> MASVIKPTQYKPVPDEEPNSTDVEETLERIKNNDPKLEEVNLNNIRNIPIPTLKAYAEALKENSYVKKFALANTRADDHVAFAIAIMLKANKTITSLNLDSNHITGKGILAIFRALLQNNTLTELRFHNQRHICGGKTEMEIAKLLKENTTLLKLGYHFELAGPRMTVTNLLSRNMDKQRQKRLQEQRQAQ

Tropomodulins (Tmods) constitute a conserved family of four isoforms that work in conjunction with one of several tropomyosin (TM) isoforms to cap the pointed end of actin filaments in cytoskeletal structures characterized by their uniform distribution of the lengths of actin filaments. Leiomodins (Lmods) are related to Tmods, and constitute a subfamily of three isoforms: Lmod1, expressed preferentially in differentiated smooth muscle cells; and Lmod2 and Lmod3, expressed more abundantly in skeletal and cardiac muscles89101112. Lmods are distinguished from Tmods by the presence of a C-terminal extension, featuring a proline-rich region and a WH2 domain. We show that ABS2, and not the C-terminal extension, is the main factor distinguishing Lmods and Tmods as filament nucleators and pointed-end-capping proteins, respectively.

To test this hypothesis we designed Tmod–Lmod ABS2 hybrid constructs aimed at combining their respective pointed-end-capping and nucleating activities. The first two constructs (TL1ABS2 and TL2ABS2) consisted of Tmod1 residues 164–229 and Lmod1 residues 365–486 (or Lmod2 residues 246–367). Strikingly, at 25 nM both TL1ABS2 and TL2ABS2 had nucleation activities comparable to that of their full-length Lmod counterparts, albeit at higher concentrations the full-length proteins displayed higher activities. Importantly, both TL1ABS2 and TL2ABS2 had much higher activity than the wild-type ABS2 domains from which they originate. The structure of TL1ABS2, the strongest of the hybrid nucleators, was determined at 2.1 Å resolution, and shows Tmod1 residues Glu-177 to Phe-229 followed by Lmod1 residues Ala-365 to Gln-486. The structure superimposes well with those of Tmod1ABS2 (r.m.s.d. of 0.41 Å for 125 equivalent Cα atoms) and Lmod1ABS2 (r.m.s.d. of 0.27 Å for 124 equivalent Cα atoms). What is more, the side chains in the hydrophobic core of TL1ABS2 have the same rotamer orientations as in the two parent structures. Therefore, the strong nucleation activity of TL1ABS2 is solely due to its amino-acid composition, and not to changes in the overall structure. Curiously, the hybrid constructs combining the capping N terminus of Tmod1's ABS2 with the added affinity of Lmod's ABS2 were better nucleators than those of the wild-type proteins. The ABS2 of Lmod has the required affinity to recruit two or more subunits for nucleation, but by adding a pointed-end-binding element, we have limited the ability of this domain to bind along the length of the filament when in isolation, that is, the hybrid constructs emphasize nucleation at the expense of filament side-binding. These constructs constitute the smallest single-domain protein with strong nucleation activity identified thus far.>[2x]GAMAGVFTYETEFTSVIPPPRLFKAFILDADNLIPKIAPQAVKCAEIIEGRGGVGTIKKITFGEGSQFGSVTHK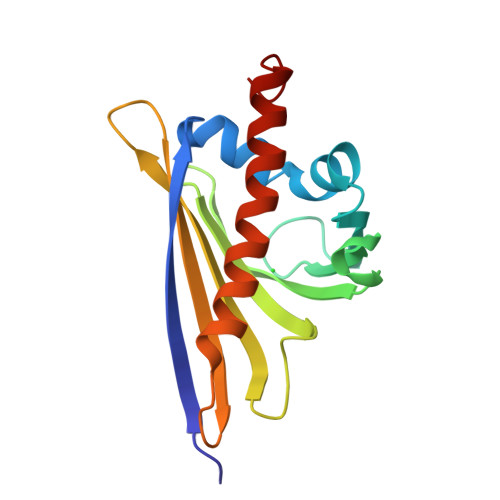IDGIDKENFVYSYSLIEGDALSDKIEKISYETKLVSSSDGGSIIKSTSNYHTKGDVEIKEEHVKAGKEKASHLFKLVEGYLLANPNEYC> MALSDADVQKQIKHMMAFIEQEANEKAEEIDAKAEEEFNIEKGRLVQTQRLKIMEYYEKKEKQIEQQKKIQMSNLMNQARLKVLRARDDLITDLLNEAKQRLSKVVKDTTRYQ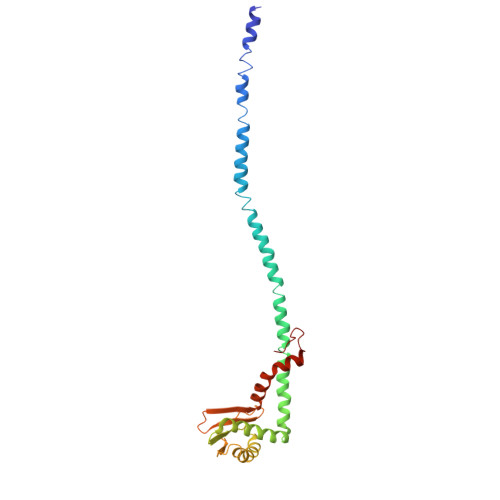VLLDGLVLQGLYQLLEPRMIVRCRKQDFPLVKAAVQKAIPVYKVATKRDVDVQIDQEAYLPEEIAGGVEIYNGDRKIKVSNTLESRLDLIAQQMMPEVRGALFGANANRKFLD>GDDSDILNSTAADEVTAHLAAAGPVGMAAAAAVATGKKRKRPHVFESNPSIRKRQQTRLLRKLRATLDEYTTRVGQQAIVLCISPSKPNPVFKVFGAAPLENVVRKYKSMILEDLESALAEHAPAPQEVNSELPPLTIDGIPVSVDKMTQAQLRAFIPEMLKYSTGRGK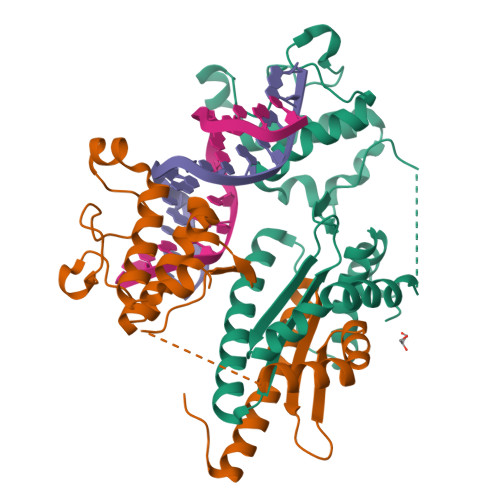PGWGKESCKPIWWPEDIPWANVRSDVRTEEQKQRVSWTQALRTIVKNCYKQHGREDLLYAFED[2x]> MAEKAQFYYPGETDVAENRRKYMNPNYELKKLREIPDEDIVRLMGHREPGEEYPSVHPPLEEMEEPECPIRELVEPTEGAKAGDRIRYIQFTDSVYFAPIHPYIRARMYMWRYRGVDTGSLSGRQIIEVRERDLEKIAKELLETEIFDPARSGVRGATVHGHALRLDEN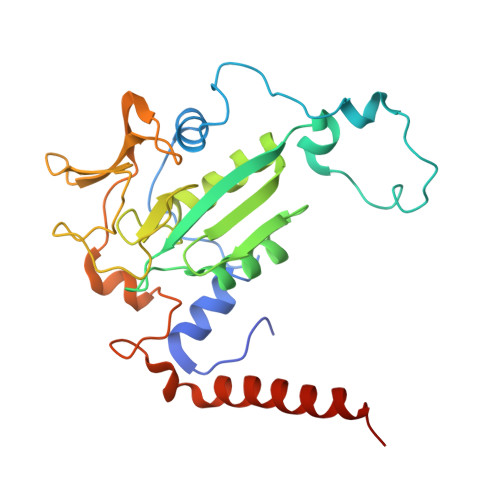GLMLHALRRYRLNEETGEVEYVKDQVGIELDEPIPVGAPADEDDLKERTTIYRIDGTPYREDEELLQVVQRIHELRTLAGYRPEEAEGK Ciliary motility is regulated by the conserved nexin-dynein regulatory complex (N-DRC), which links adjacent doublet microtubules and regulates and coordinates the activity of outer doublet complexes. The N-DRC is a large 1.5-MDa, ~50-nm-long Y-shaped complex with two main regions: the base plate and linker regions. The N-DRC bridges neighboring DMTs and restricts sliding motions between DMTs. Here, using cryo-electron microscopy in conjunction with biochemical cross-linking and integrative modeling, we localize 12 DRC subunits in the N-DRC structure of Tetrahymena thermophila.

In this study, we revealed the molecular architecture of the N-DRC of T. thermophila by an integrative modeling approach. Importantly, our data identified an additional N-DRC component, DRC12. Loss of DRC3 in the drc3 mutant strain led to the loss of part of the distal domain (based on our study, the distal domain lost in the drc3 mutant represents DRC9/10 complex). We propose DRC3 binds to DRC4 first, leading to the assembly of DRC9/10 heterodimers. As a result, DRC4 plays a crucial role in assembling the N-DRC distal domain. Regulatory signals can be sent to dynein e through the N-terminus of DRC9. In addition, DRC10 may send signals to dynein g through DRC3. Therefore, the DRC9/10 coiled-coil may be the important regulatory hub in the N-DRC that regulates dyneins g and e by receiving the signal from CCDC96/113. In active cilia, the N-DRC linker region is not well observed by cryo-ET, probably because of its flexibility.

> MNPSQTQKGKIQIQVSRGSIDLLVRTMYEDINNIKLKNERFQKKKRAEDERRRRERYAEIQQEAIASGKKNAALEMKWAELKELDECEELNREMQDQQQTFQQIIEGKENLRKEFEEELKRKDDEYVKMLKEQSNDIKDMISKMRSQFYKIRDANMQELEDIERHFEQERSNLLNEFKAKIQATFKKHLDLEEQYVKEHAKTEEEQTKNIEDLRIKGAKHYAELKITMETEIQDLEKCFEDMKALYQLITEKLDYSLKVLQEKFHENNSMCDELKRKENNFKNRLKQLTKDYKQYDKKFKLENKNLTQEYKRIIRQFKELQKKFKHFEKADLDKYSEIQKMNEAEVKELKDKIIKCNITIHIQQLGMQWIPPQSEEEILAQQKLQLEQGGKAEEEEEREFEFCISEIKIGEICNIILEEADFLIDDKLREELEGSAEPEQIFQRLDCIKKCLYIDSEDEMNLFFRELITKCRVKSAEEIEEEARKQLLLLGLIKEAEENENPEGEEVQQQEGAQQKKKEEGNKKDDPKGKEGAKDSKENANPQGQNKSNQDERKKKKDGQDDHAGQGQGQYDSNQGGMGENQEEGENAEGQENLEGEIEKEIDLENTQINLNEVVKFLQNWQANKDKRKEKLEKESSKKAVKQETEREKKERIAREGKKYWEKLTQVLPERTFRIWNVNFFKFSFEKQILLNQINKLRFWTDLCPNIMNFFWTDKNQSKKPVNCITKMKNQRIFQINTYKLIMNLLSALQDSLIQIKDKDDFIQTKISTNLFTFHNFQILLQIFIVNQSFLFIRLCQSYSKKIILLIKNINQKLFNLSNFKNQFSF;> MALLGKTLKGRSTRPGGIPQKRNIKWRQLAKNQEEFDQLKQLAKMKREGLKARIKDEQKVVTFNKKKLITYWRKIMRIAKTEQLKNEIDIYSQNNQRELDSKEAFIQMLDKNLDEAEDQFQIALRNHLIHIENLMQLQEARMRGLAEEFNRDVNILETEFDLEREEMVKTHKTQLKELEDMIETVKEEDKKKTEEAQNEFSQFKEETKNKNLEETNVMKIILETKQTKYYTELEQMNSKFQSDTSNKVKDHQFYHAHNKNRKQEIDRYLRTISSKKAKIDLMKLKILQHCKEFNARNSALKKEKENISRNYHELKLKMQKFREEESRRLKELSNNSRNAVLKLREYCALGEKILKTAELCRRLETEKEKVLPFYESSVDEDQIPEQLKNEFEHLKKEDAEEYAYLNNFYKRYNKVLLDKLAIEKQKENLQRDNQLLKSLLKQYLDGISLNDDVLKNENNPLLVVNHKFNLGKMPVEKIENKTVIEGVFEVRNTSHQLQGQRAPPFQ;> MSNYISNYVQSTIVTKTVQNKDKKTGKNSVDPRVINEQLILDAVKQFNQENNKITTENIILQQLRQLQLSFKNILKIQHLQGLERLEKLQLDNNIIEKIENIDHLVNLKWLDLSFNCIKKIEGLDKLKELTDLSLFNNYIEKIEGLHNNTKLNVFSIGNNRLKSYEEITLYFGYKPRGEEGTNDRPEFKRLQVLNVSGNPFTKDKENEYKNHIICAIPNLKYLDYVFIDEGDRQLIRQDEQISNSYNFTTTDYYQQMQAQEQKEEMDRQTLKKKKDARMDILDNLKDEYLKIEDLQRVKIIKPNQINEEIEKYCGKINDHVVEMQAAVIQKHQLILQEMSKTEVSYKEQEALHEKETLQILKEFEHEKKVEFRNWEKEAANGDAKKEESRLKTLLQKTTSLKNKLMDIEIQLVEELEAIFTDYDTKKKETAWKDIEEIIVLGQKKIEEENVKFYSNLNVIKNKEEANYNSTQQQQLEEENNEEDDEKASLLENKEQLAQMIGNIKETLIDSHTKIILSAQMELQKDLAEYAKQQKNKMYERNRKNISQIIAQIDAYQTEINEKLKQGDDESDHEN;> MSKAAKAKKNVPVVSKLEADARKAAEGVNDNESEEFKKAMRKEARALVEQFNEEKKLLAFYQQERQKINYNWIIAKKELEDKKSELINKEREIQDLQENHFMTLNVYKQKIKHLLFQNQDQQSELKKDVEVTLKQLEDQHRIKSRELKTDVRSLKVTKKEQEISQQDYLFALKSEHDKQMTLMRQDYERQVNDIKRKYDLKMQNLTKEMEEARAAMIKQLEDNKNQKIAEIIKEHTQKYNDIKNYYSEITATNLDYRKTLKNEIKELQTKDEEYKKTLQQTEKGYKELNEPLQALGIEIIQLKKQDEEQEAIIKEKEELKQKIDNQERLFRKLEYEYEVKLQQFQYLERERNALYAKFNQTVFEIHQKSGLENLILEKKVTNLREDLEIKDLQIHQVLTAANIDPNSVGSINKSLEEVESLKNELISELQAQLKQIRKAHSHMVKAYEGKLSEFVIPVEELGFDPLVPTNTD;> MPPKKAKGKKKKEEEPDDEYKSMTGADLTQTLEKLKERVNEMRTNRNYIQMDRDMVENFYHNTLKEISEVKTKISNKETEAEEKESKHRIDVKVFLQKVKHLEYEQEKSNLNIEDDGKKAKEKEDAYFEDITKNMKQLKTQLKSEYLEKEKANIQQVQEEKKDHQSLLKIQQKKFDELINNLIIKYEERLAKLKEDLELKLKVEIHELEERKNLHINELMNNHEKAFAELKKYYNDITAENLNLIKAHKEKIAQIYANIQLNTKNVADNQAKNEQLKEPLAKHREIRNKLKEDLKQFAKHKMSLQNLKSKAITLKDKITKLERDGKDLDEKYEKVVREKQELEKKFEDITQEVKKNADLNNNVLSNRLQILLKEYNNKEEELRTIIDNAGLDHNLHEQLKQRVQQSIEAKNTLIKNLKYSIHHATKAYNDAIRVYEAKLVEFGIPIEELGFQPLETITSSMPAGLVSS;> MLAKKLALARSQGKPDPFKKDEFPLLQHIAVEVVSQNYILYPDLKGVPENVRDTIISKITTDLDILTMAPNIDQESFWQRACKNRWEKSQKSINIEEHGRSWKVAYLERYMEEFLTNIQNADDPNKKQILQAELKAAASWIHTLNLQNINQNIDIDFICKYLPLLTSLTLTYGTKYSGMDYNKQSVGMKLSEAANLGEAIKNCYSLLSLNISANMIDDDLLRFIMAGVNMNISLIELNLSHNKIEDQGARRIAKFLMRNEILLYLNLGNNLIGYEGSRYLAQALKVNKNLQSLNLKLNNLGDKAGKKLFQDLMLNKTLLELDVSGNQFEFETALKLSDYVADSMCGLKVLNIANNDFNDSCYENLKTGFTKNYSLAKLDLRGNKFSKTQEEKEQELKDPFRMFNLSQTEKELTQIIIRHDLTAQKIQFFSESDLDKIKQLKELQGAKQEPEKVIQQDQNKE;> MGDKKGKKKGGGEEDESTLQLSRQYKKKCELNGINPSKLFKEKLDFAVEEDENIEKIHLWEELGPVGVRSIMDSLTEIPYLHTKSIRLWKVKAQDEGTRTICNYMEKSKTIEYLDLMDNQVGSLGCEFLGRVLHPQIEIPLLKLKLDHNEFGTEGLMQLAAGLCMNSVLEKLSLNYCAITAEGSKYIQQILSFVNTNLKKLKMKGNLLKNEGVHQLFRAFKVNKTLEKVDLSDNQFDTTLGDDQDPEANPNFFETNKDAIEHNKQIIENICEVLKAADTLLYYDFRFNNISKTDAKAIIDCLEANKNIYYMELSEHIPKDLIERKKGLMKKRKPKKKKKKKAKKK;> MDHNEGGYSHHQIEGQEGQQQQAPVGGGGEDIFQVLENITQVQNEKLKRCQEFKEQENIPRQYIENSPKEELVLEHVIQFKRQFQYQLYYEDKRDLFLYPKNECDVYKFICTTIRPTKLGFLELYDYQQCSKYLSEFVQYEELDPPNEFPLVIPSPTNVAVWQKGDCFDMSILLCSLLIGVGYDAYCVYGKAPREITTRNESLMECLFLEKGKYIEENDKKPKQTLEQNENALLKKPIAHSKWDQTQETKAREAEEEKRRIALTINDDEPDELLEDPYQGQRVHCWVLLRSGKRDVQQNIFIEPSTGRMYSPSTCPYECVDAVFNNLNFWINMKPECEVKNLNFEEMDSSLNWEYVMLDTLLFNKGNGNDEEGNENIDDPLNKQAQRDPEQEQLQDIAQLLDMPPPWPPKIYIDKEKFLMGTPLGEGTVYYNKVKVDNYAPYSQPDGLVQKITIFQDYKRLKVKEYRYFYKHRSDKLSIRRRYPFEFKTIEEYEPQKYENKTIPQALQQWRQVIQIDRHLRIIKYYHNRNHDGLIERVEQIGEKTMMFYQNRDDRVIYRSIRFDNKRAPSSQNNDKVFQDNHVGDVQITKMTQKFEKNPHYPANEQIQKMVIDLIKDKVIVYYHMNDGEITPIVKIYPRDSMHGFAKLNEPGGDNKIDDPLVQLENTKMVNLEKDCLNQLKQQEKIARDDEKTIREGEIRLEKTLYDKARDRFKESSKKNDDDLAKDAAASDYLYPYLEKRKLLGVSEINAQVAMEIKNEVMQKLKERLLSRAEIIQRRLEEQRQVLEQKEAQVAKRQEIDPKQEEEIRDINFKIDILEQRALRFESMALQKYEEMDNRLNKDARLAALHRK;>[2x]MYDPNTSQTEKQKQEEFLKLKIQEAFNLFVKDKKGIVDKREIPYIMRYLGQFPSEAQVRDAILPEIEEDEPSEFIKYSKFEPYMLKVLKEREYEPDDPEALLAAFKLLDQEGKGYIEIDMMKTFLEKQGIEFREQETKSFIEFATNKDPNATVIYYEDYISRLQAFTDKHIESVMKGYNNFQVKK;> MNQIDAHKLTIILRDATERLTFLDTINRQDDLSSELAGYEISKLLKKQKNLENQYADLVQLRTSLTGIQNKKNLIETQTKIVDVAQNLKESTKKLCRLFKENPDLESDALKVKKDRIQFMAVIEQLIQMVQNNSLTKFQSMTTLELEDQDRLRKLIFREKELYQEIKKLQFDRNQENKEYDNEQKDTNLKIQNLKERLLYKKARAQLKNQYKEKEARAEEGTQQRMYEFEQKQLKEKINNLKQKTDTENMVHEQLRNFLIEKEDQIKQKSDEWAKKVETCREQLQEEIDRLTVEKEKKQEELRELRERDQKEQEEKDRRERQELEEADRKQQEELDQIRLDNAIKLIQIEYQEWKDAGGGKKKRKKGKKKKK;> MQNLSKMQSRLHPRPEGEGGGGGGRTKEKGKSLQETHKEMLKNIESTNIGKPTIVEAQRILKIIDNLSTNLTIFIYLDSELISKFLDVAKHSKLSKDLVSKLSQRCLDLLKSQAEIEAKFKPYASLLDQSNKEAEDVEEEKMIDAERLRMQLENNFKDLVRHLRNSPEDFEIIKSMKTNVNPDLNDLVHCIHCQKVIMLKKLSTASEEDENHKAQLRDLEEKIEELEKKKNKIQEDLTKLKEHRQKFSKEKKEELEKLKNEIAEVKAEKEKKASQLKNELDNRLKQLERDHLAKKDKLDKELQKLEDDFAKLKQDHANDETKLKTNKRQQQNSLADNIESYDALMKDQHQKKQEIEEELAKIIEEVDTLKQLFKEIDEEKQRERELEEEFRLKKEQWEIQERRKKEAARCILHFLMARKEKSKKKKKKKGKKKK;> MSNMMYNMKWQEAINDLMEQVTLEYLPLEQNEQQLGMKYKRDSSEWFHFWATLYIKYIDIYKKLEDCYDQLVHPQKRVLLKEMLENVIVRLCETKSQVVKYNTQYDATYKSDYPNLDELVMDLKLTPDCLDIPIPRYFREEDKKRLDERNQILDALLLEYTDTKEPQEEQYEDQNTLQADMDTAIRIIQRYERGRQGIERANLAKILKKEEEKKLERQKKLAEGTEIGEETEKDDAALVIKKYWRGYKSRKLVQDIREEELLFLGMKKVVEDPTLPESQYKQAQNKRQKMKYIQEEHEQEFNDEIENLKRLVKGNEGPDILDKMRAERREWIMRELEKNEFKEAPQDPSEFYNQQVMDPEQQAAEAAKAAEEAKKKGAAKKDDKKKKGKPSELDEFLENNKPTGPSPIVLKLQEQIEKHSGEWSKRDETNNFEQKHETELAKMLIKPVVEEQIKQQVDEMIAEELDIVRLRYDIKKKKQKKPPRPRNKGKNKKKFPGDSSNKGRDPKDILAGLVEKRVAKKLIPASLMDLKGEQNVLGKIQEIQADENLKKTEALTDAKLKKAQLEEPSTKMPDPSIAQIRQIIAEYIAFPLGSKYAKEKLDKMNYFFFMGPRGSGKTLAVRALAHECNAIVLDISPSNIDGQYTDKKQIDGMINSAFKVAKEFQPAIIYCEDFEYIFGQAKKKKSQVNPLFAKMKKPLMDFKKGKFFEPEDRVVFIGSTNRPWDCSQKEIKSFFDKKIYFPFPNYGTRMLLFKTFLEQKKVPLPDNFPINTIAHITEGWSAGSFKMAIDRVFTERRLQKINEEQIKLSEFIGPLSNVPFTSKEEFKEFKKFNQVVTGLQANYEAKKAPADDQKGDKNKKKK;> MASEDGEMPSQFEGIDPEQLTESQMQQYMMEMQRQGLLDSNMEGGQYEEGYEEGQEGEGYGEEYGDQDYDGNQNEYDSQQDSQQQGHDQVNEMHQDRYDRRVNSEISGNYEADDETLRKIRRDLLDNINLERRHRDLQPVYIDLTTNNISQYYSEYLVNNEHNQDFYENAKVRYNNLGECELCHITAKFEPDADITKEYIYDYFMEIGYLFLESEEEKRIILNPANNHIGIGVFFDEIQIVVVLILSEKVLCIQKISQPEQNKIEIRGKMLDENFGIYAIRIMNVDDQKKDIKGVGPEFIEYTRSTQEWMASFELELYNQDRMAIEYYTRVSPDSIPYKKKQSKNEKLTYKHLQLRLRTPFQIYPDPKYAAEDEKERIRKEQEILAHEEQERKEREENDAKRLKQSRKDYGDGQYDDDEHGQDDFNSQSDISDKDKHHDSMHAEQEQNQQAAQQQQDTISNKEIRQELEMAITEAQRQHDEFMLQNHKLQEEIKLLKNKNDGFVDRSNETAMNEHKYLNTLAHVHQIRLDLKQTQTRYNQMSQELQKKLEQKQKKCNEIKYAFLELKREVAKKAANSRTDKPIPEQQINEWEKAELQKSKELQELRLQILRLRNAYVKNQKILKKKEELAEGLHLIDFEQLKIENQTLNEKIEERNEELHKLKKKNTTTIQILTHTREKLGFVQGENGELNSQNVRKDQELDDMRKQLTQQKKTKDKLRSVNLTLKQQTGIVNSEELGQDYRDLRTRVSKLEEEKKRLEQKLRSMHEAIKTANQISTQNMQSQNNSLKKPYQPY;>[2x]MDNTGKLEKQLVTLNDGLPKKPAKEIIEELKHHLYQDFQKFFSEEKKQQYQNNFALFDRDNDKYINLSELKELLTSVNITFPDDELEELYNEFCLTSPEADGINEDAVFIIVSKKIRDNDKDEQLTQAFKLVEKAVNDELAKTPNETKEQEGYIRVEQFKELLMTLGNRWSEEQANEFLKDINPKSDERINYLDVVKKLMKR;>MSKKSGKGKGKNDGDELGAEKEQVLRTKVESLIQRLGHEQERADRAKAAENELRARLFDLDKDFKNEKDRLFSITSDMTRQYKQMQDELLNQVNDLNKTVIEKDEEIKKKDQQIQDMTKDYEYKLKKKDDEIQDLKRKIEEMSAEFAKMLKDTLDKMQERIEMVQWDSDTDPQMMKRLKDMTGLSNN[2x]>[4x]MAWPKVQPEVNIGVVGHVDHGKTTLVQAITGIWTSKHSEELKRGMTIKLGYAETNIGVCESCKKPEAYVTEPSCKSCGSDDEPKFLRRISFIDAPGHEVLMATMLSGAALMDGAILVVAANEPFPQPQTREHFVALGIIGVKNLIIVQNKVDVVSKEEALSQYRQIKQFTKGTWAENVPIIPVSALHKINIDSLIEGIEEYIKTPYRDLSQKPVMLVIRSFDVNKPGTQFNELKGGVIGGSIIQGLFKVDQEIKVLPGLRVEKQGKVSYEPIFTKISSIRFGDEEFKEAKPGGLVAIGTYLDPSLTKADNLLGSIITLADAEVPVLWNIRIKYNL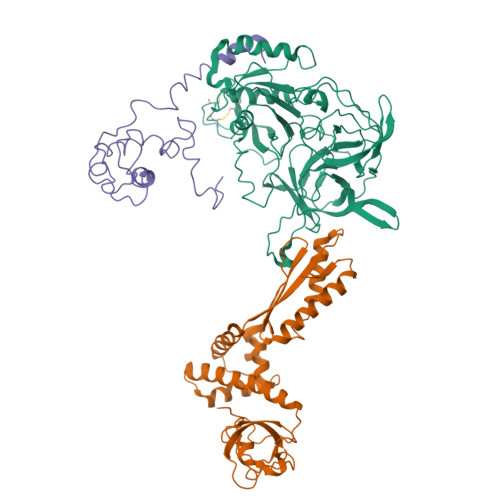LERVVGAKEMLKVDPIRAKETLMLSVGSSTTLGIVTSVKKDEIEVELRRPVAVWSNNIRTVISRQIAGRWRMIGWGLVEI;>MIYSRSKLPSEGEILIATVKQVFDYGSYVSLDEYGGLQAFLPWSEVSSKWVKNIRDVLKENRKVIVKVIRVDRRKGTVDVSLKKVTDDERRKKNLQWKKIQRLDKILELVSQKLKLSEKDAWEQVAWKLEAKYGDPITAIEKAVKEGEKILIDAGVPEIWVKPLLEEASKHAEERKVKMSGLITVRTNEPLGVEKIKEVISKALENIEQDYESLLNIKIYTIGAPRYRVDVVGTNPKEASEALNQIISNLIKIGKEENVDISVVKK[4x];>MSSEKEYVEMLDRLYSKLPEKGRKEGTQSLPNMIILNIGNTTIIRNFAEYCDRIRREDKICMKYLLKELAAPGNVDDKGELVIQGKFSSQVINTLMERFLKAYVECSTCKSLDTILKKEKKSWYIVCLACGAQTPVKPL[4x]>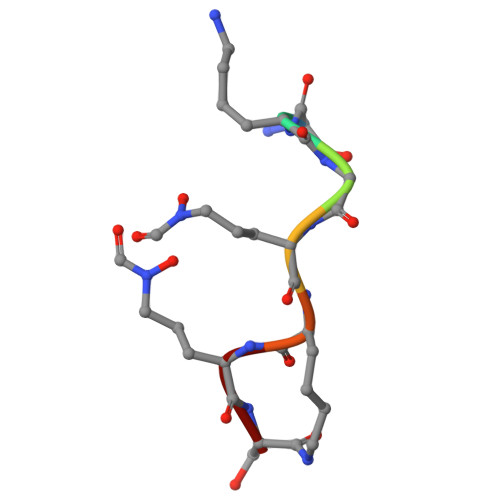 SKGKKKS>MLVSVYLALLVACVGQAHSQANLMRLKSDLFNRSPMYPGPTKDDPLTVTLGFFLQDIVKVDSSTNEVDLVYYERQRWKLNSLMWDPNEYGNITDFRTSAADIWTPDITAASSTRPVQVLSPQIAVVTHDGSVMFSPAQRLSFMCDPTGVDSEEGVTCAVKFGSFVYSGFEIDLKTDTDQVDLSSYYASSKYEILSATQTRQVQHYSCCPEPYIDVNLVVKFRERRAGNGFFRNLFDENLYFQGHHHHHH[5x]

Protein-engineering methods have been exploited to produce a surrogate system for the extracellular neurotransmitter-binding site of a heteromeric human ligand-gated ion channel, the glycine receptor. Acetylcholine-binding protein is a highly conserved ortholog of the pLGIC extracellular ligand-binding domain (ECD) with properties similar to nAChR. Mutations affecting key residues in the orthosteric agonist site at the α1(−)/β(+) interface affect the potency of both activation by glycine and inhibition by strychnine. We therefore set out to generate a high-fidelity surrogate of this α1(−)/β(+) orthosteric binding site using the 2α1:3β stoich­iometry [Fig. 1(a)] by exploiting protein-engineering methods and the thermal stability of acetylcholine-binding protein from Aplysia californica (AcAChBP). Ultimately, the highly stable AcAChBP framework has allowed us to introduce nine amino-acid substitutions that have resulted in a stable surrogate for a heteromeric neurotransmitter site that binds glycine.

Variant I incorporated five changes: T53F, Q74R, Y110A, I135S and W164F. The key observation from the structure of the variant I strychnine complex concerned the Y110A, W164F and I135S substitutions. Trp164 NE1 donates a hydrogen bond to the carbonyl of Ile135, thus linking two β-strands from different subunits. The electron density of the phenylalanine (Phe164) was poorly ordered, perhaps as the reduction in the side-chain size of an adjacent residue (Y110A) opened up one side of the binding site, allowing a greater degree of conformational freedom. Neither variant I nor variant II appeared to be able to bind nicotine. The combined Y110A and I135S substitutions may open up the binding site such that nicotine can longer bind in an optimal fashion. Variants I and II presented structural features consistent with site-directed mutagenesis and electrophysiological data that suggest interacting roles for specific residues.> MRVTELIIDGFKSYAVRTVITGWDESFNAVTGLNGSGKSNILDAICFVLGITNMSTVRAQNLQDLIYKRGQAGVTKASVTIVFDNRDKKRSPIGFEEYATISVTRQIVLGGTTKYLINGHRAQQQTVQNLFQSVQLNINNPNFLIMQGRITKVLNMKPAEILAMIEEAAGTRMFEDRKEKALKTMAKKDLKLQEITELLRDEIEPKLEKLRQEKRSGGSGGSMNMIDSVEKKEMSLKHMMKTVLKDKHKIEETIATLDEYKRKALQETWEKVNGDFGQIFNELLPGSFAKLEPPEGKDLTDGLEVKVRL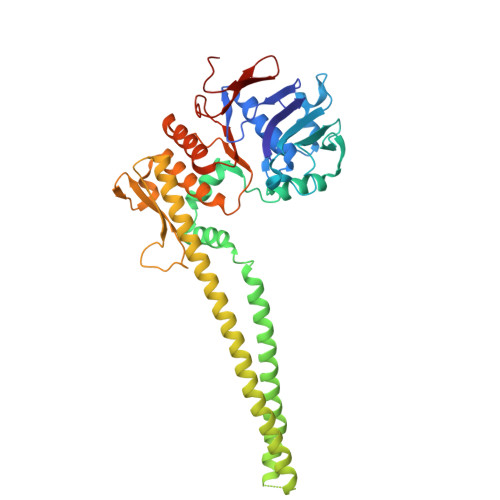GKVWKQSLTELSGGQRSLIALSLIMALLQFKPAPMYILDEVDAALDLSHTQNIGRLIKTRFKGSQFIVVSLKDGMFQNANRIFRVRFSEGTSVVQALTPADLK>[2x]GMGKRILLLEKERNLAHFLSLELQKEQYRVDLVEEGQKALSMALQTDYDLILLNVNLGDMMAQDFAEKLSRTKPASVIMILDHWEDLQEELE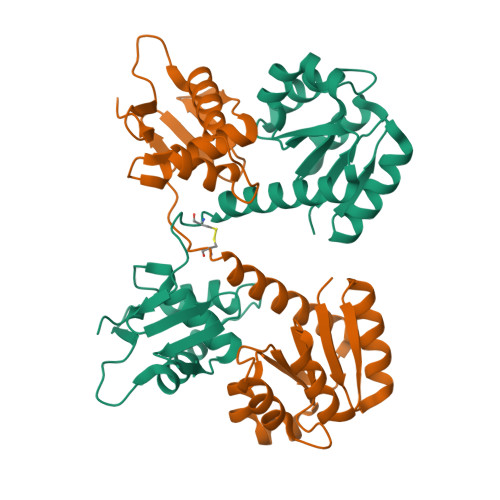VVQRFAVSYIYKPVLIENLVARISAIFRGRDFIDQHCSLMKVPRTYRNLRIDVEHHTVYRGEEMIALTRREYDLLATLMGSKKVLTREQLLESVWKYESATETNIVDVYIRYLRSKLDVKGQKSYIKTVRGVGYTMQEG> MLGRIWLPVLIVVAVAAGALIVMNVRTVFGSNPVVVTEKTSDNAEDFNPKVVTYEIFGSGSSAVINYMDLEGMPQRVESTPLPWSLTLQTTLPSVMPHIMAQGDGDSITCRVTVDDVVKEE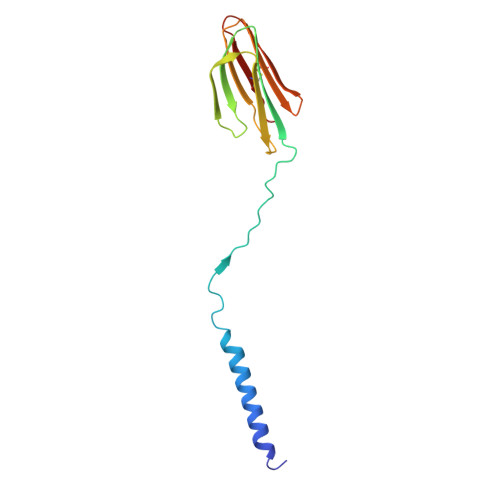RTATGMNAETFCYVKAA> GSHMYEYPVFSHVQAGMFSPELRTFTKGDAERWVSTTKKASDSAFWLEVEGNSMTTPTGSKTSFPDGMLILVDPEQAVEPGDFCIARLGGDEFTFAKLIRDSGQVFLQPLNPQ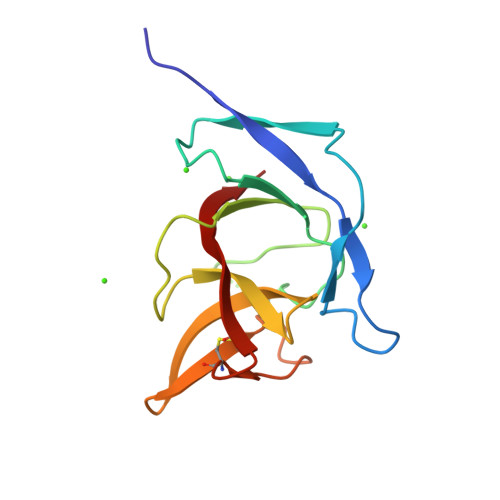YPMIPCNESCSVVGKVIASQ>QQMGRGSMSKIVKIIGREIIDSRGNPTVEAEVHLEGGFVGMAAAPSGASTGSREALELRDGDKSRFLGKGVTKAVAAVNGPIAQALIGKDAKDQAGIDKIMIDLDGTENKSKFGANAILAVSLANAKAAAAAKGMPLYEHIAELNGTPGKYSMPVPMMNIINGGEHADNNVDIQEFMIQPVGAKTVKEAIRMGSEVFHHLAKVLKAKGMNTAVGDEGGYAPNLGSNAEALAVIAEAVKAAGYELGKDITLAMDCAASEFYKDGKYVLAGEGNKAF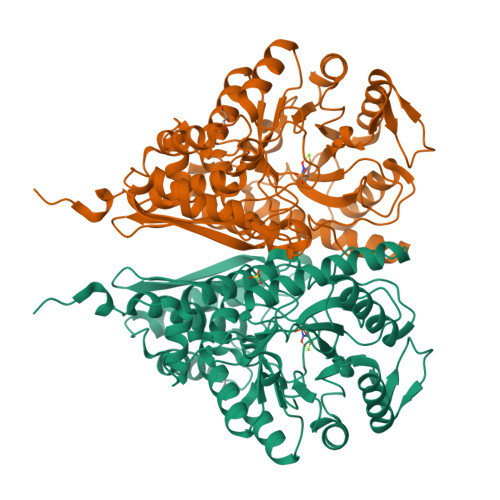TSEEFTHFLEELTKQYPIVSIEDGLDESDWDGFAYQTKVLGDKIQLVGDDLFVTNTKILKEGIEKGIANSILIKFNQIGSLTETLAAIKMAKDAGYTAVISHRSGETEDATIADLAVGTAAGQIKTGSMSRSDRVAKYNQLIRIEEALGEKAPYNGRKEIKGQA[6x]>MSVQRLSLGAARCLSAGVARVQASQALVAQKAVAVAPTRAQAAPAEVAQVRSMSVLAASKMVGAG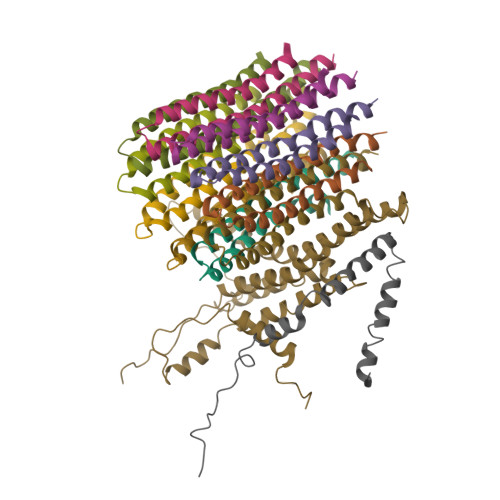CATIALAGVGAGLGVMFGSLINGAARNPNIAKQLVGYALLGFALTESIALFSLLVVFLILFA[10x];> MSVLSSVSMGSRIGSSLLGRSSAYLAQCGFSTRSNLNGSIDTSSSVFQALSSDNENKPAASPLNVKLPGMSCSSILLPKTSRIAVPFGNQTMAMSSVRDVKTGSLPTNFLTGVYRFWRSQNPAEKPHDPVNDRLLPAVVDASDKRASIGTWATTFFCTIISCNLLGLMPFNEAPTSGLGFATGLGVSVWATATILGLSKTGFKFPGHFIPGGTPWPMAFIFVPLETISYTFRAVSLGVRLWVNMLAGHTLLHILTGMALALPFSLGFFSMVPATFGVCCLLSALVGLEYLVAVLQSGVFSILSTVYVGEFNHDKFIGPAAKIVKKIH;> MMLRTLTRSSAVAGQAVRLFKTSAAAAEGNSVAGIIKSVNETSGANLLSSLKTIKAQAAPIYPAAASSTGYSTQAKIALFGALSWILYRADGQSKAHEWIVDLNLNVLQAAWLISFSSLIPFRAVYFAFRGMAPATASTLNGLKTFSSISL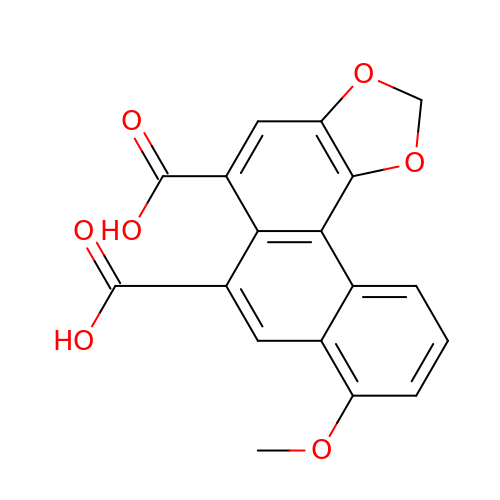8-methoxyphenanthro[3,4-d][1,3]dioxole-5,6-dicarboxylic acid | C18 H12 O7 | KTEBZKXXNMHJFH-UHFFFAOYSA-N>[4x]MDVRRTPTPTTLTQYIIKSQPPHSRGDFTLLMMAIQTSVKVIEKNIRRAGMKGMLGYIAGQSANATGDHQAKLDVISNIAFKAYLLSSTSVCVLGSEEEEQMIIAESGRRGDYLIFFDPLDGSSNIDANVSVGSIWGVWRLPKDTTINSVEDANAVIRMLKGTDMVSAGYAVYGSATNLVLTSGHGVDGFTLDPNIGEFILTHPHISI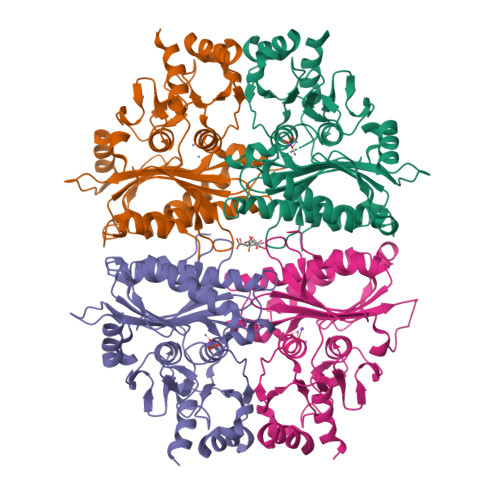PKKRSIYSVNEGNYGKWEPWFKEYIDYLKMNKTTRYSARYIGSMVGDIHRTLLYGGIFCYPKDANQVEGKLRLLYEAAPMAMIVEQAGGKAVGSNGRILEQSITRLHQRTPVYFGSRQEVDLCMAFRDRNVKTEALAPTSSKL> EDSLGMEVGYRLIPMVDFQQDGELLGRIRSIRKKFAQDMGFLPPVVHIRDNMDLQPARYRILMKGVEIGSGDAYPGRWLAINPGTAAGTLPGEKTVDPAFGLDAIWIESALKEQAQIQGFTVVEASTVVATHLNHLIGQFSAELFGRQEAQQLLDRVSQEMPKLTEDLVPGVVTLTTLHKVLQNLLAEKVPIRDMRTILETLAEHAPLQSDPHELTAVVRVALGRAITQQWFPGNEEVQVIGLDTALERLLLQALQGGGGLEPGLADRLLAQTQEALSRQEMLGAPPVLLVNHALRPLLSRFLRRSLPQLVVLSNLELSDNRHIRMTATIG;> MYTASGIKAYAQVSVESAVMSASPHQLIEMLFDGANSALVRARLFLEQGDVVAKGEALSKAINIIDNGLKAGLDQEKGGEIATNLSELYDYMIRRLLQANLRNDAQAIEEVERLLSNIAEAWKQISPKASFQESRGTASGAGGSEGGGSEGGTSGATEDSDYATEVSNMSRAQILQQAGTSVLAQANQVPQNVLSLLR

Type III secretion systems (T3SSs) are membrane-embedded nanomachines that export dedicated proteins from the bacterial cytoplasm. FliD and FliC are found in complex with their dedicated chaperones FliT and FliS, respectively, in the cytoplasm. Here we report the structures of the ternary complexes among the FliD and FliC flagellar proteins, their cognate chaperones FliT and FliS, and the export gate protein FlhAC. FlhAC folds in a clamp-like structure with four discrete subdomains (d1 through d4).

Similarly to FlhAC−FliT−FliD, NMR analysis showed that the highest quality spectra were yielded by a ternary complex formed between FlhAC and a fused construct wherein FliCC was covalently linked to FliS. The structure of the FlhAC−FliS−FliCC ternary complex was determined by X-ray crystallography at a resolution of 2.6 Å. All contacts within the ternary complex are formed between FliS and FlhAC, with FliC making no direct interaction with FlhAC. Two distinct binding interfaces mediate complex formation. The most significant appears to be the juxtaposition of the FliS N-terminal helix (α1) with the FlhAC hydrophobic cleft located between the d1 and d2 domains. The binding interface buries a total surface of 680 Å2. In addition, a hydrogen bond is formed between the hydroxyl group of FliS Tyr10 and FlhAC Asp456. Amino acid substitutions that perturbed the binding interface decreased the ternary complex stability, with FliS residue Tyr10 and several FlhA residues in the binding cleft being essential for complex formation. FliS−FliC and FliS−FliCC (where FliCC is a construct consisting of residues 454–495) have the same affinity for FlhA indicating that the first 156 residues of FliC do not contribute to FlhA binding. Specifically, FliS Tyr10 and FliT Tyr106 interact very similarly with the FlhAC cleft and the Tyr residue is absolutely conserved in both FliT and FliS.> SSSTKKTQLQLEHLLLDLQMILNGINNYKNPKLTRM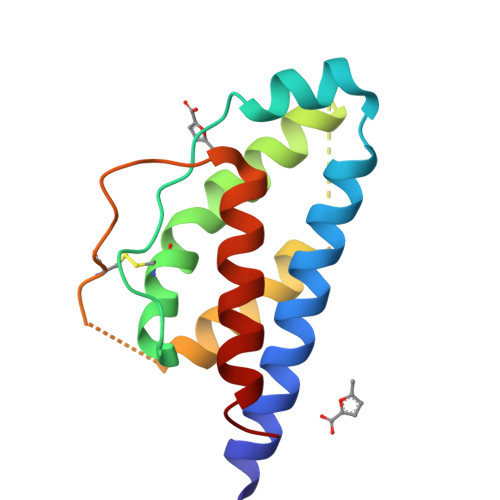LTFKFYMPKKATELKHLQCLEEELKPLEEVLNLAQSKNFHLRPRDLISNINVIVLELKGSETTFMCEYADETATIVEFLNRWITFSQSIISTLT>MTDGLNQLYNLVAQDYALTDTIEALSRMLHRGTIPLDTFVKQGRELARQQFLVRWHIQRITSPLS[2x];>[2x]GAMDISQLFHDEVPLFDN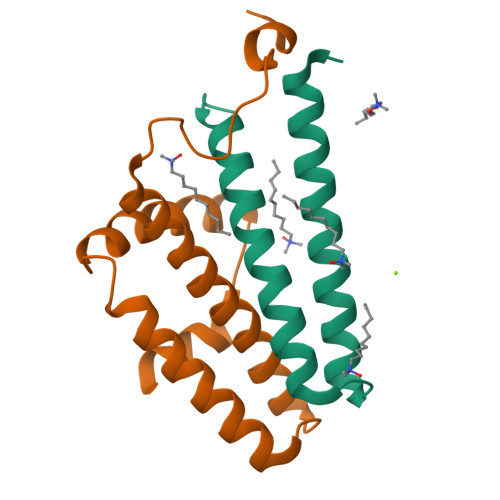SITSKDKEVIETLSEIYSIVITLDHVEKAYLKDSIDDTQYTNTVDKLLKQFKVYLNSQNKEEINKHFQSIEAFADTYNITASNAITRLERG The FimH type-1 fimbrial adhesin allows pathogenic Escherichia coli to adhere to glycoproteins in the epithelial linings of human bladder and intestinal tract, by using multiple fimbriae simultaneously. Pauci- and high-mannose type N-glycans are natural FimH receptors on those glycoproteins. The lectin domain of the fimbrial adhesin FimH from E. coli recognizes with the highest affinity and in monovalent fashion oligomannose-3 and -5 N-glycans. Hereby, we describe the conversion from monovalent- to bivalent N-glycan binding to the FimH lectin domain, with two full N-glycan structures, namely α1,6-fucosylated oligomannose-3 (Man3Gn2F1) and oligomannose-6 (Man6Gn2).

To visualize the interaction between FimH and core-fucosylated oligomannose-3, we have performed cocrystallization and obtained a crystal structure at 1.4 Å resolution. The ligand Man3Gn2F1 interacts with FimH via its α1,3-arm, and the mannose binds in the monosaccharide-binding pocket (M) of FimH via the conserved ligand residues Phe1, Ile13, Asn46, Asp47, Tyr48, Ile52, Gln133, Asn135, Tyr137, and Asn140. The two glycans, Man3Gn2F1 and Man3Gn2 respectively, interact with FimH via the Manα1,3Manβ1 disaccharide, oriented in the mannose-binding pocket of FimH in a similar way. The interaction created with Manα1,3Manβ1,4GlcNAc is therefore the same for the two ligands and allowed to maintain the potential hydrogen bond between O6 of GlcNAc 2 and the hydroxyl group of Thr51. The α1,6-fucosylated N-acetylglucosamine 1 in one of the FimH monomers of the asymmetric unit has a very high motility and was modeled in two alternate conformations, altA and altB. In one FimH monomer, the larger Man3Gn2F1 ligand samples more space, by rotating around the GlcNAc 1–GlcNAc 2 glycosidic bond (torsion angle ψ), resulting in at least two alternate conformations. On the other FimH monomer, two fucoses are close in the crystal packing and take on the altB conformation near the side chain of Tyr137. Core α1,6-fucosylation of oligomannose-3 does not change its binding through the α1,3-linked mannose arm. The preference of FimH is markedly selective for the α1,3-linked mannose branch of α1,6 core-fucosylated oligomannose-3, identical to what was found for oligomannose-3 without fucose. That is interesting, because the crystal structure of FimH in complex with Man3Gn2F1 confirmed previous data on Man3Gn2 binding, in that the chitobiose moiety (GlcNAc 2–GlcNAc 1) gets priority over Manα1,6Manβ1 (4′-3) for interactions with FimH in the monovalent binding mode in their competition for the same space.

>[2x]FACKTANGTAIPIGGGSANVYVNLAPVVNVGQNLVVDLSTQIFCHNDYPETITDYVTLQRGSAYGGVLSNFSGTVKYSGSSYPFPTTSETPRVVYNSRTDKPWPVALYLTPVSSAGGVAIKAGSLIAVLILRQTNNYNSDDFQFVWNIYANNDVVVPT> MRGSHHHHHHGSLVPRGSMRVLLIEKNSVLGGEIEKGLNVKGFMADVTESLEDGEYLMDIRNYDLVMVSDKNAL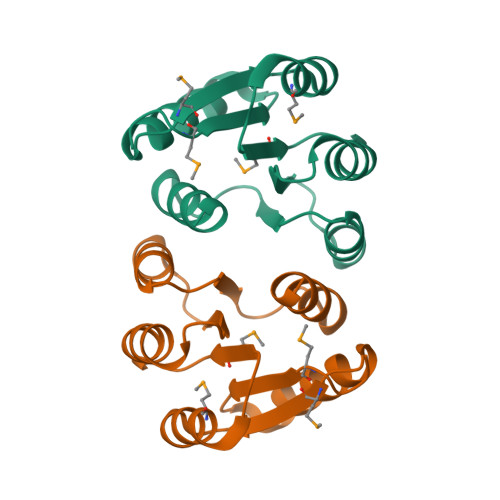SFVSRIKEKHSSIVVLVSSDNPTSEEEVHAFEQGADDYIAKPYRSIKALVARIEARLRFWGSN>[4x]GIGPVADLTITNAAVSPDGFSRQAVVVNGGTPGPLITGNMGDRFQLNVIDNLTNHTMLKSTSIHWHGFFQKGTNWADGPAFINQCPISSGHSFLYDFQVPDQAGTF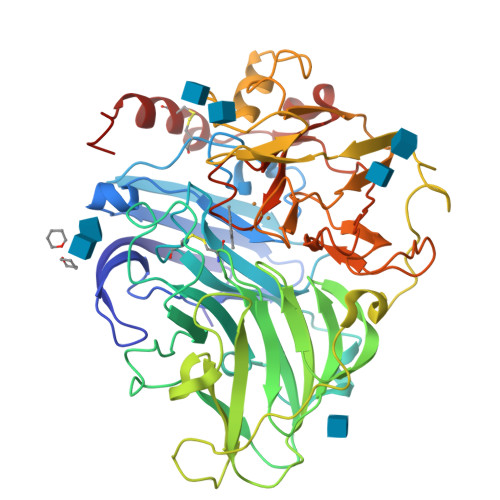WYHSHLSTQYCDGLRGPFVVYDPNDPAADLYDVDNDDTVITLVDWYHVAAKLGPAFPLGADATLINGKGRSPSTTTADLSVISVTPGKRYRFRLVSLSCDPNYTFSIDGHNMTIIETDSINTAPLVVDSIQIFAAQRYSFVLEANQAVDNYWIRANPNFGNVGFTGGINSAILRYDGAAAVEPTTTQTTSTAPLNEVNLHPLVATAVPGSPVAGGVDLAINMAFNFNGTNFFINGASFTPPTVPVLLQIISGAQNAQDLLPSGSVYSLPSNADIEISFPATAAAPGAPHPFHLHGHAFAVVRSAGSTVYNYDNPIFRDVVSTGTPAAGDNVTIRFRTDNPGPWFLHCHIDFHLEAGFAVVFAEDIPDVASANPVPQAWSDLCPTYDARDPSDQ>[2x]DDDQVAFSFILDNIVTQK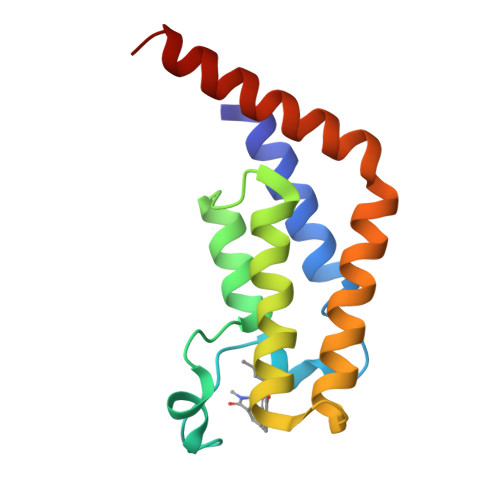MMAVPDSWPFHHPVNKKFVPDYYKVIVNPMDLETIRKNISKHKYQSRESFLDDVNLILANSVKYNGPESQYTKTAQEIVNVCYQTLTEYDEHLTQLEKDICTAKEAALEEAE>[8x]GTGAMWLTKLVLNPASRAARRDLANPYEMHRTLSKAVSRALEEGRERLLWR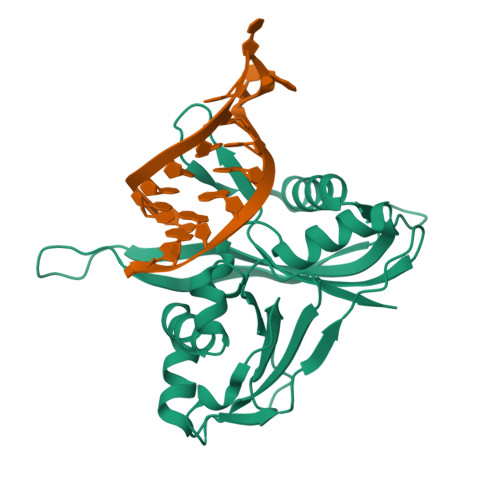LEPARGLEPPVVLVQTLTEPDWSVLDEGYAQVFPPKPFHPALKPGQRLRFRLRANPAKRLAATGKRVALKTPAEKVAWLERRLEEGGFRLLEGERGPWVQILQDTFLEVRRKKDGEEAGKLLQVQAVLFEGRLEVVDPERALATLRRGVGPGKALGLGLLSVAP The self-splicing group II introns are bacterial and organellar ancestors of the nuclear spliceosome and retro-transposable elements of pharmacological and biotechnological importance. Besides catalyzing their self-splicing, group II introns also act as mobile retroelements, thus crucially contributing to genetic diversity throughout evolution. Integrating enzymatic, crystallographic, and simulation studies, we demonstrate how these introns recognize small molecules through their conserved active site. These RNA-binding small molecules selectively inhibit the two steps of splicing by adopting distinctive poses at different stages of catalysis, and by preventing crucial active site conformational changes that are essential for splicing progression.

To mimic a more physiological conformation of the active site immediately after 5’-exon hydrolysis, we thus co-crystallized OiD1-5 (the free intron) with the 5’-exon-like oligonucleotide 5’-AUUUAU-3’ in the presence of Mg2+ and K+, and we solved the X-ray structure of this complex in the absence of inhibitors, and in the presence of intronistat B or the di-brominated intronistat B derivative ARN25850 at different soaking time (1 h or 2.5 h). Interestingly, after 2.5 h soaking the crystal structure of OiD1-5 co-crystallized with the 5’-exon-like oligonucleotide and with intronistat B also reveals an Fo-Fc omit map compatible with the binding of both oligonucleotide and inhibitor in the active site (highest contour value = 4.0 σ, volume of the peak at 3.0 σ = 301 Å3). Unexpectedly, though, this volume is oriented differently from the volume occupied by intronistat B after 1 h soaking and in the exon-free state (RSCC = 0.90). The structure shows that the group II intron active site still recognizes the compound’s pyrogallol motif through M1 (1.9 Å from intronistat B O22 atom and 2.1 Å from intronistat B O24 atom), M2 (1.9 Å from intronistat B O24 atom and 2.2 Å from intronistat B O26 atom), and its conserved catalytic residues, i.e. the catalytic triad and the 2-nucleotide bulge. Interestingly, in this structure, the nucleotides around the splice junction also contribute to the recognition of the compound, i.e. U0 [3.3 Å between intronistat B O22 atom and U0 O3’ atom and 3.1 Å between intronistat B O24 atom and U0 O3’ atom] and U2 (weak 3.9 Å contact between O18 of intronistat B and O4’ of U2). However, in this structure intronistat B has lost its interaction with A181 in the EBS1 site (15 Å between O18 in intronistat B and N1 in A181), which is now based-paired to its cognate 5’-exon nucleotide U0. Similar to the free intron structure, also in the presence of the 5’-exon the two catalytic M1-M2 ions coordinate the compound and are stabilized at a distance dM1-M2 = 4.01 ± 0.46 Å.

> GUGUGCCCGGCAUGGGUGCAGUCUAUAGGGUGAGAGUCCCGAACUGUGAAGGCAGAAGUAACAGUUAGCCUAACGCAAGGGUGUCCGUGGCGACAUGGAAUCUGAAGGAAGCGGACGGCAAACCUUCGGUCUGAGGAACACGAACUUCAUAUGAGGCUAGGUAUCAAUGGAUGAGUUUGCAUAACAAAACAAAGUCCUUUCUGCCAAAGUUGGUACAGAGUAAAUGAAGCAGAUUGAUGAAGGGAAAGACUGCAUUCUUACCCGGGGAGGUCUGGAAACAGAAGUCAGCAGAAGUCAUAGUACCCUGUUCGCAGGGGAAGGACGGAACAAGUAUGGCGUUCGCGCCUAAGCUUGAACCGCCGUAUACCGAACGGUACGUACGGUGGUGUGG;> AUUUAU ClpP is a highly conserved protease regulated by ATPases in bacteria and in mitochondria. In bacteria, ClpP is responsible for modulating the expression of virulence factors, antibiotic resistance, and the formation of biofilms and persisters. Likewise, Homo sapiens ClpP (HsClpP), which is found in the mitochondria, is a key protease regulating mitochondrial proteins homeostasis. The dysfunction of ClpP by small molecule activators has recently been demonstrated to be a possible method of discovering antibacterial and anticancer drugs.

Incorporation with the isoleucine fragment and 4,4,4-trifluorobutyl motif into the core scaffold of ICG-001 provided a potent ClpP activator ZG180. ZG180 is more potent than ICG-001 in activating SaClpP for α-casein hydrolysis, as evidenced by a 3-fold decrease in EC50. However, ZG180 also promotes HsClpP for α-casein hydrolysis, which indicates that ZG180 is also a global activator for both bacterial and mitochondrial ClpP proteins. Either ZG180/SaClpP or ZG180/HsClpP structure is a single tetradecamer composed of two stacked heptameric rings. Like the previously characterized ClpP activators, the binding of fourteen ZG180 molecules induces an open-gated state in the tetradecameric ClpP cylinders with an enlarged axis entrance pore. The apparent electron densities in the 2fo-fc and fo-fc omit maps unambiguously demonstrate ZG180 binding on the apical surface of SaClpP and HsClpP. The naphthyl motif and trifluorobutyl chain in ZG180 form hydrophobic stacking in the binding pockets of SaClpP, which contributes to the enhanced interactions. A network of hydrogen bonds between ZG180 and the side chains of D27, L49, Q52, Y61, and Q89 collectively increase the binding affinity to SaClpP. While SaClpP and HsClpP share a high similarity in the primary sequences, there is a large indole motif of W146 in HsClpP but a much smaller isopropyl side chain of I91 in SaClpP in the conserved position. Indeed, structural superimposition of the ZG180/SaClpP and ZG180/HsClpP complexes also reveals that the α-carbon of the naphthyl motif in ZG180 is likely to be a discriminant site for introducing steric clash against the bulky side chain of W146 in HsClpP.

>MNLIPTVIETTNRGERAYDIYSRLLKDRIIMLGSQIDDNVANSIVSQLLFLQAQDSEKDIYLYINSPGGSVTAGFAIYDTIQHIKPDVQTICIGMAASMGSFLLAAGAKGKRFALPNAEVMIHQPLGGAQGQATEIEIAANHILKTREKLNRILSERTGQSIEKIQKDTDRDNFLTAEEAKEYGLIDEVMVPETK[14x]>[3x]NNPYLFRSNKFLTLFKNQHGSLRLLQRFNEDTEKLENLRDYRVLEYCSKPNTLLLPHHSDSDLLVLVLEGQAILVLVNPDGRDTYKLDQGDAIKIQAGTPFYLINPDNNQNLRILKFAITFRRPGTVEDFFLSSTKRLPSYLSAFSKNFLEASYDSPYDEIEQTLLQEEQEGVIVKMP;>[3x]MQLRRYAATLSEGDIIVIPSSFPVALKAASDLNMVGIGVNAENNERNFLAG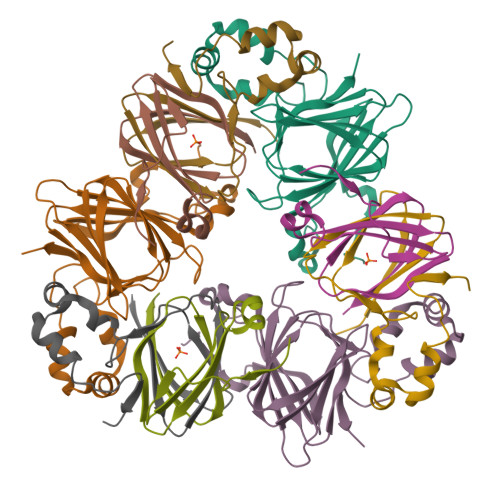HKENVIRQIPRQVSDLTFPGSGEEVEELLENQKESYFVDGQP;>DKPFNLRSRDPIYSNNYGKLYEITPEKNSQLRDLDILLNCLQMNEGALFVPHYNSRATVILVANEGRAEVELVGLEQQQ[3x]>METIIHKIRLFDVAQADAFEFWVQNVDYATCPDLPSVVRFDVHRASLQANAPYHYVEVIKITDRAAFDADMETSTFAGLVQAFSRMAEVVEE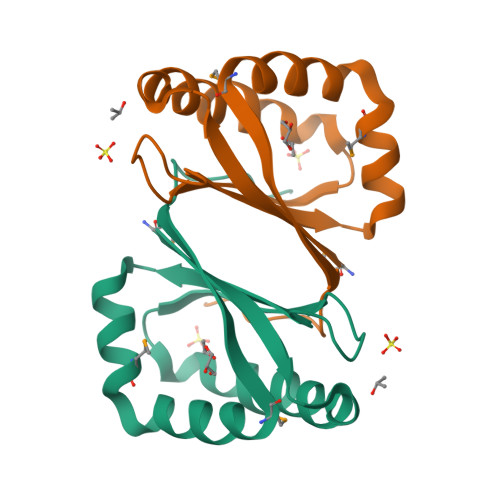LAGEQLGSGYAAG[2x]> GPLGSPEFIEKSFVI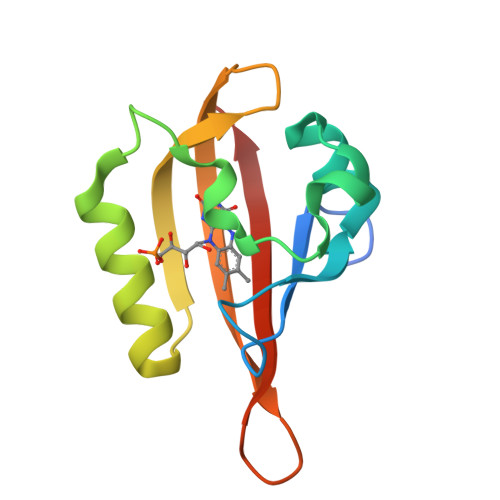TDPRLPDYPIIFASDGFLELTEYSREEIMGRNARFLQGPETDQATVQKIRDAIRDQRETTVQLINYTKSGKKFWNLLHLQPVRDRKGGLQYFIGVQLVGSDHV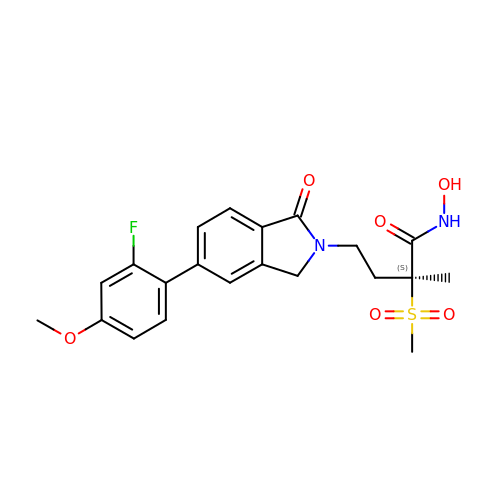(2~{S})-4-[6-(2-fluoranyl-4-methoxy-phenyl)-3-oxidanylidene-1~{H}-isoindol-2-yl]-2-methyl-2-methylsulfonyl-~{N}-oxidanyl-butanamide | C21 H23 F N2 O6 S | BYDRVBMZUCDIRW-NRFANRHFSA-N>[2x]GSDWSKPLPPSERLEQELFSGGNTGINFEKYDDIPVEATGNNCPPHIESFSDVEMGEIIMGNIELTRYTRPTPVQKHAIPIIKEKRDLMACAQTGSGKTAAFLLPILSQIYSDGPGEALRAMKENGRYGRRKQYPISLVLAPTRELAVQIYEEARKFSYRSRVRPCVVYGGADIGQQIRDLERGCHLLVATPGRLVDMMERGK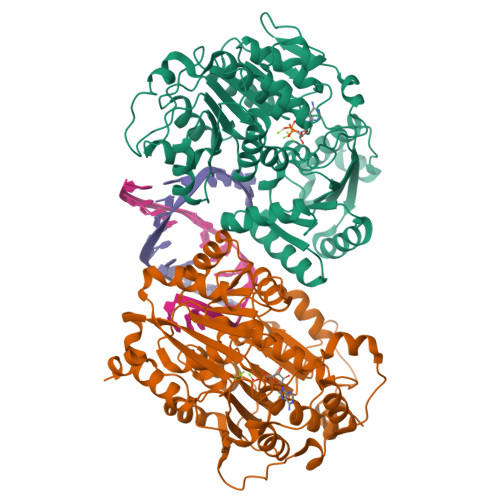IGLDFCKYLVLDEADRMLDMGFEPQIRRIVEQDTMPPKGVRHTMMFSATFPKEIQMLARDFLDEYIFLAVGRVGSTSENITQKVVWVEESDKRSFLLDLLNATGKDSLTLVFVETKKGADSLEDFLYHEGYACTSIHGDRSQRDREEALHQFRSGKSPILVATAVAARGLDISNVKHVINFDLPSDIEEYVHRIGRTGRVGNLGLATSFFNERNINITKDLLDLLVEAKQEVPSWLENMAYEHHYKG>SVDTMALWLGLRAVLVVAGLAVLLQLIRGWLSSKSYVFNREEIARLAKEHSGLDYEVAFSKIIVELRKKHPGHILQDEDLQWVFVNAGGWMGSMCLLHASLTEYVLLFGTAVDTGGHSGRYWAEISDTILSGTFRQWKEGTTKSEIFYPGDTIVHEVGEATSVQWSSGTWMVEYGRGFIPSTLAFALADTIFSTQDFLTLFYTVKVYSKALLLEASTHLSQLGFF[12x]

The sigma-1 receptor (σ1R) is a non-opioid transmembrane receptor which has been implicated in many diseases, including neurodegenerative disorders and cancer. The sigma-1 receptor (σ1R) is a small, unique integral membrane receptor that is localized primarily in the endoplasmic reticulum (ER). σ1R responds to a structurally diverse array of synthetic ligands such as (+)-pentazocine (agonist) and haloperidol (antagonist). Published structures of human σ1R reveal its homotrimeric organization of a cupin-fold β-barrel body that contains the ligand binding site, a carboxy-terminal V-shaped two-helix bundle, and a single amino-terminal transmembrane helix, while simulation studies have suggested a ligand entry pathway that is generated by conformational rearrangements of the cupin-fold domain. Here, we present multiple crystal structures, including an open-like conformation, of σ1R from Xenopus laevis. Together with functional binding analysis our data suggest that access to the σ1R ligand binding site is likely achieved by protein conformational changes that involve the carboxy-terminal two-helix bundle, rather than structural changes in the cupin-fold domain.

In our continued search for an open structure of xlσ1R, crystals with an appearance (cube-like) different from the xlσ1Rclosed-endo crystals (cuboid-like) were obtained and their structure was determined to 3.56 Å (xlσ1Ropen-endo). The xlσ1Ropen-endo structure was solved in the P212121 space group, with each asymmetric unit containing 12 protomers. Similar to all σ1R structures, xlσ1Ropen-endo also assembles as homotrimers. Each asymmetric unit contains four trimers, which are packed in a tetrahedron shape through the α1–α1 contacts. Structural comparison between xlσ1Ropen-endo and xlσ1Rclosed-endo shows that the two structures are very similar, with the exception of two regions. One region consists of the transmembrane helix α1, which swings ~18° away from the trimer center in xlσ1Ropen-endo compared to xlσ1Rclosed-endo. In xlσ1Ropen-endo, the α4 helix rotates slightly away from α5, and the side chain of Tyr203 from α5 adopts a gauche+ χ1 rotamer to point to the cupin-fold domain, thus creating an opening between α4 and α5 that generates a direct pathway for the ligand from the outside milieu to the ligand-binding site. Therefore, the xlσ1Ropen-endo structure may represent an open-like conformation for σ1R and is consistent with PATH2 that predicts the ligand entry between α4 and α5. Like xlσ1Rclosed-endo, the xlσ1Ropen-endo crystals were grown in the absence of any known ligand, but the xlσ1Ropen-endo structure also has an unidentifiable electron density within its ligand-binding pocket.[azanyl-[4-(trifluoromethyl)phenyl]methylidene]azanium | C8 H8 F3 N2 | 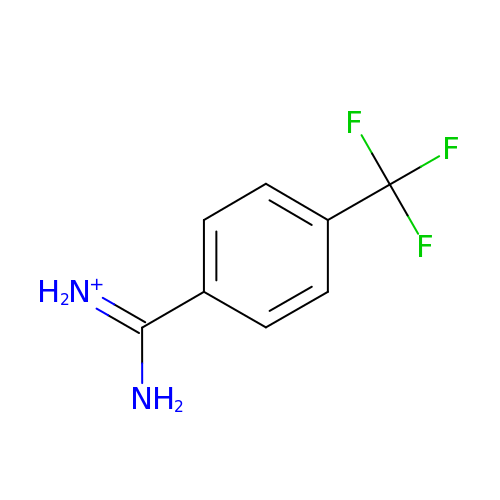XFLGYXVBXUAGQV-UHFFFAOYSA-O N,N'-BIS(2-AMINOETHYL)-1,2-ETHANEDIAMINE 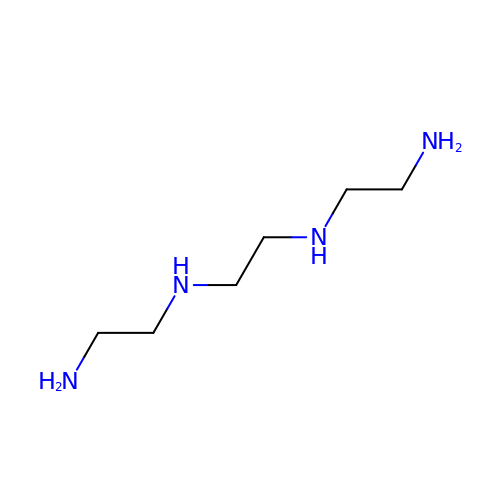| C6 H18 N4 | VILCJCGEZXAXTO-UHFFFAOYSA-N>MSGRLTGKVALVSGGARGMGASHVRAMVAEGAKVVFGDILDEEGKAMAAELADAARYVHLDVTQPAQWKAAVDTAVTAFGGLHVLVNNAGILNIGTIEDYALTEWQRILDVNLTGVFLGIRAVVKPMKEAGRGSIINISSIEGLAGTVACHGYTATKFAVRGLTKSTALELGPSGIRVNSIHPGLVKTPMTDWVPEDIFQTALGRAAEPVEVSNLVVYLASDESSYSTGAEFVV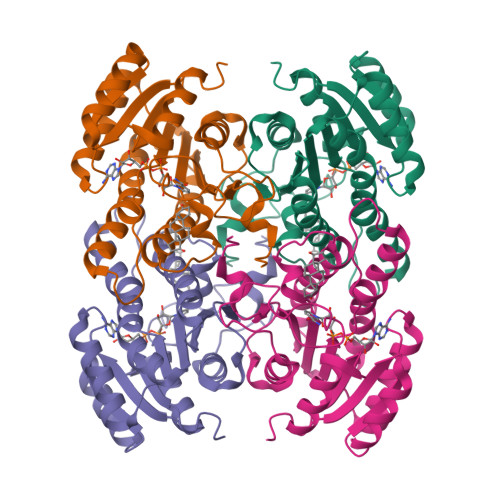DGGTVAGLAHNDFGAVEVSSQPEWVT[4x]> GSHMISEHDSVLEKYPRIQKVLNSTVPALSLNSSTRYEGKIINIGGTIIKARLPKARIGAFYKIEPSQRLAEVIAIDEDEVFLLPFEHVSGMYCGQWLSYQGDEFKIRVGDALLGRLIDGIGRPMESNIVAPYLPFERSLYAEPPDPLLRQVIDQPFILGVRAIDGLLTCGIGQRIGIFAGSGVGKSTLLGMICNGASADIIVLALIGERGREVNEFLALLPQSTLSKCVLVVTTSDRPALERMKAAFTATTIAEYFRDQGKNVLLMMDSVTRYARAARDVGLASGEPDVRGGFPPSVFSSLPKLLERAGPAPKGSITAIYTVLLESDNVNDPIGDEVRSILDGHIVLTRELAEEN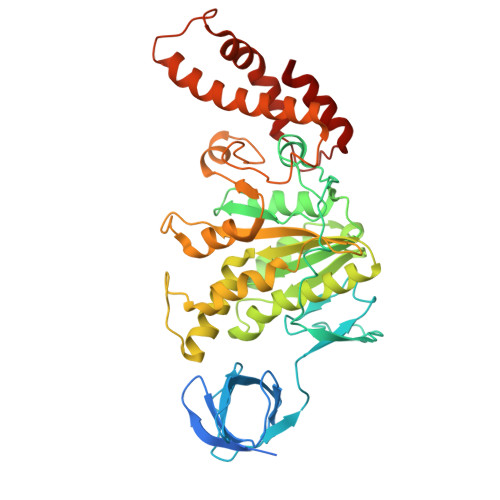HFPAIDIGLSASRVMHNVVTSEHLRAAAECKKLIATYKNVELLIRIGEYTMGQDPEADKAIKNRKLIQNFIQQSTKDISSYEKTIESLFKVVA HEXADECA-10,12-DIEN-1-OL | C16 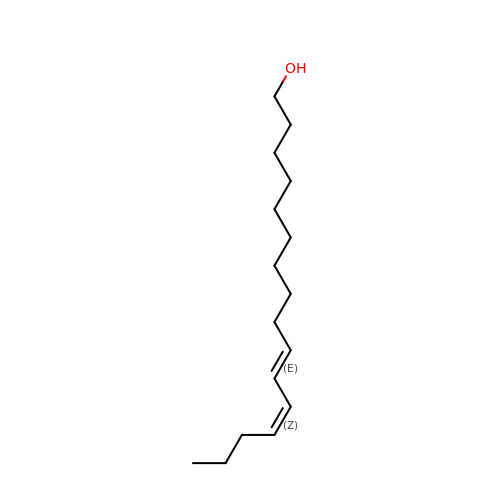H30 O | CIVIWCVVOFNUST-SCFJQAPRSA-N>[4x]VIPDYFKQSFPEGYSWERSMTYEDGGICIATNDITMEGDSFINKIHFKGTNFPPNGPVMQKRTVGWEASTEKMYERDGVLKGDVKMKLLLKGGGHYRCDYRTTYKVKQKPVKL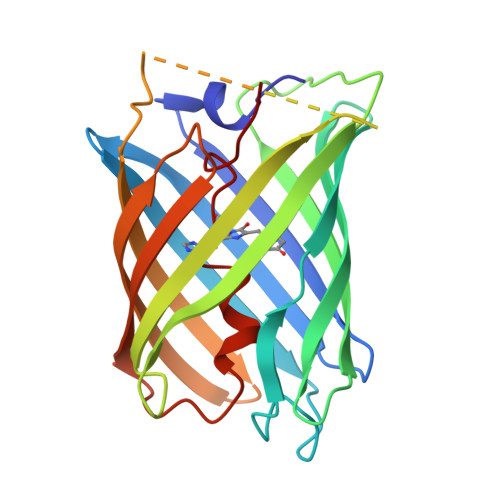PDYHFVDHRIEILSHDKDYNKVKLYEHAVARNSTDSMDELYKGGSGGMVSKGEETITSVIKPDMKNKLRMEGNVNGHAFVIEGEGSGKPFEGIQTIDLEVKEGAPLPFAYDILTTAFHYGNRVFTKYPR;>VIPDYFKQSFPEGYSWERSMTYEDGGICIATNDITMEGDSFINKIHFKGTNFPPNGPVMQKRTVGWEASTEKMYERDGVLKGDVKMKLLLKGGGHYRCDYRTTYKVKQKPVKLPDYHFVDHRIEILSHDKDYNKVKLYEHAVARNSTDSMDELYKGGSGGMVSKGEETITSVIKPDMKNKLRMEGNVNGHAFVIEGEGSGKPFEGIQTIDLEVKEGAPLPFAYDILTTAFF[2x];>HYGNRVFTKYPR[2x]> GSVDQVDARRNVPQNDPVTVVVLKATAPFKYESPENGKSTMFHATVASKTQYFHVKVFDINLKEKFVRKKVITISDYSECKGVMEIKEASSVSDFNQNFEVPNRIIEIANKTPKISQLYKQASGTMVYGLFMLQKKSVHKKNTIYEIQDNTGSMDVVGSGKWHNIKCEKGDKLRLFCLQLRTVDRKLKLVCGS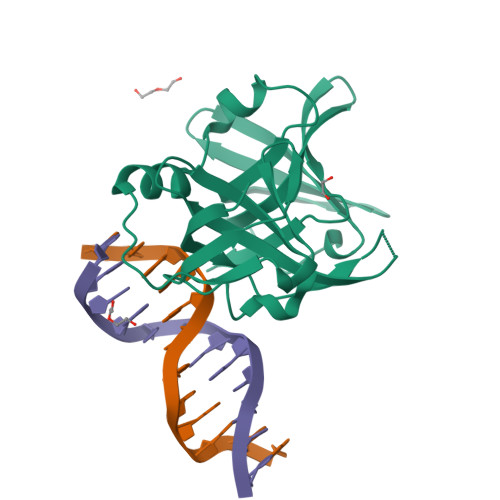HSFIKVIKAKKNKEGPMNVNAAAS> MAAAPQAPGRGSLRKTRPLVVKTSLNNPYIIRWSALESEDMHFILQTLEDRLKAIGLQKIEDKKKKNKTPFLKKESREKCSIAVDISENLKEKKTDAKQQVSGWTPAHVRKQLAIGVNEVTRALERRELLLVLVCKSVKPAMITSHLIQLSLSRSVPACQVPRLSERIAPVIGLKCVLALAFKKNTTDFVDEVRAIIPRVP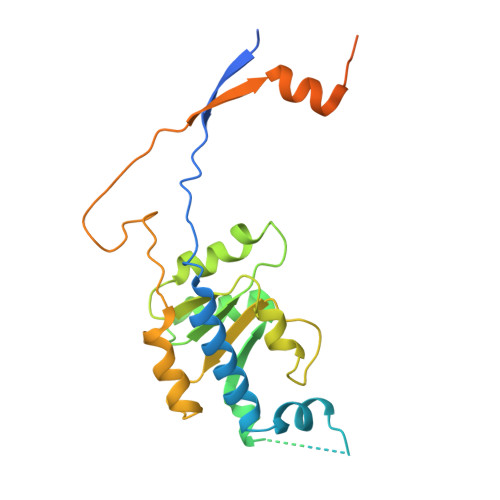SLSVPWLQDRIEDSGENLETEPLESQDRELLDTSFEDLSKPKRKLADGRQASVTLQPLKIKKLIPNPNKIRKPPKSKKATPK> MKRDHHQFQGRLSNHGTSSSSSSISKDKMMMVKKEEDGGGNMDDELLAVLGYKVRSSEMAEVALKLEQLETMMSNVQEDGLSHLATDTVHYNPSELYSWLDNMLSELNPPPLPASSNGLDPVLPSPEICGFPASDYDLKVIPGNAIYQFPAIDSSSSSNNQNQQLQSCSSPDSMVTSTSTGTQIGGVIGTTVTTTTTTTTAAGESTRSVILVDSQENGVRLVHALMACAEAIQQNNLTLAEALVKQIGCLAVSQAGAMRKVATYFAEALARRIYRLSPPQNQIDHCLSDTLQMHFYETCPYLKFAHFTANQAILEAFEGKKRVHVIDFSMNQGLQWPALMQALALREGGPPTFRLTGIGPPAPDNSDHLHEVGCKLAQLAEAIHVEFEYRGFVANSLAD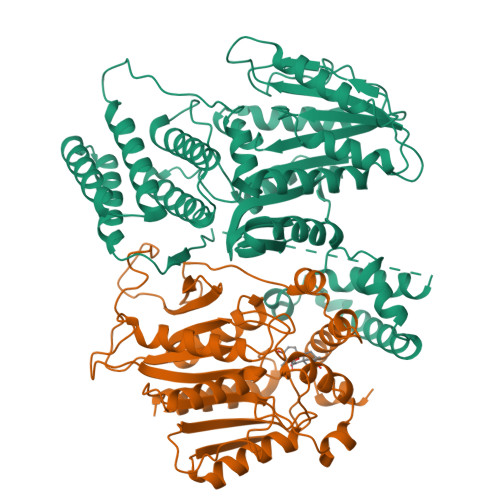LDASMLELRPSDTEAVAVNSVFELHKLLGRPGGIEKVLGVVKQIKPVIFTVVEQESNHNGPVFLDRFTESLHYYSTLFDSLEGVPNSQDKVMSEVYLGKQICNLVACEGPDRVERHETLSQWGNRFGSSGLAPAHLGSNAFKQASMLLSVFNSGQGYRVEESNGCLMLGWHTRPLITTSAWKLSTAAYGGWSHPQFER;> MAASDEVNLIESRTVVPLNTWVLISNFKVAYNILRRPDGTFNRHLAEYLDRKVTANANPVDGVFSFDVLIDRRINLLSRVYRPAYADQEQPPSILDLEKPVDGDIVPVILFFHGGSFAHSSANSAIYDTLCRRLVGLCKCVVVSVNYRRAPENPYPCAYDDGWIALNWVNSRSWLKSKKDSKVHIFLAGDSSGGNIAHNVALRAGESGIDVLGNILLNPMFGGNERTESEKSLDGKYFVTVRDRDWYWKAFLPEGEDREHPACNPFSPRGKSLEGVSFPKSLVVVAGLDLIRDWQLAYAEGLKKAGQEVKLMHLEKATVGFYLLPNNNHFHNVMDEISAFVNAECGGDYKDDDDK> MNQQKSLTL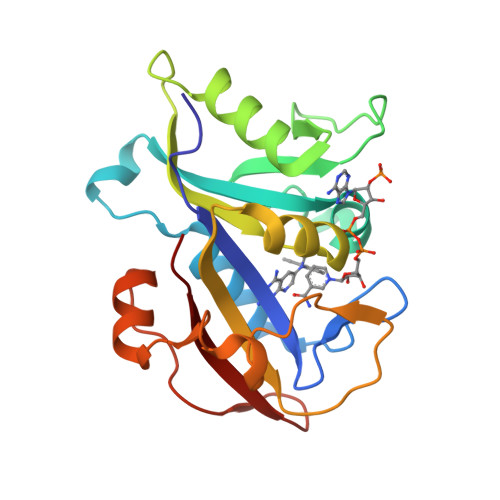IVALTTSYGIGRSNSLPWKLKKEISYFKRVTSFVPTFDSFESMNVVLMGRKTWESIPLQFRPLKGRINVVITRNESLDLGNGIHSAKSLDHALELLYRTYGSESSVQINRIFVIGGAQLYKAAMDHPKLDRIMATIIYKDIHCDVFFPLKFRDKEWSSVWKKEKHSDLESWVGTKVPHGKINEDGFDYEFEMWTRDL>[3x]MPMFLPCVLVPNTRDCRPLTYQAAIPELRTPEELNPIIVTPPIQAIDQDRNIQPPSDRPGILYSILVGTPEDYPRFFHMHPRTAELSLLEPVNRDFHQKFDLVIKAEQDNGHPLPAFAGLHIEILDENNQSPYFTMPSYQGY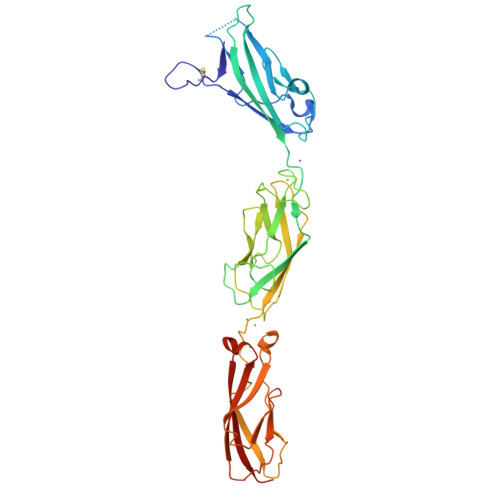ILESAPVGATISDSLNLTSPLRIVALDKDIEDVPPSGVPTKDPELHLFLNDYTSVFTVTQTGITRYLTLLQPVDREEQQTYTFSITAFDGVQESEPVIVNIQVMDANDNTPTFPEISYDVYVYTDMRPGDSVIQLTAVDADEGSNGEITYEILVGAQGDFIINKTTGLITIAPGVEMIVGRTYALTVQAADNAPPAERRNSICTVYIEVLPPLEHHHHHH1-(2,3-dihydroindol-1-yl)prop-2-en-1-one 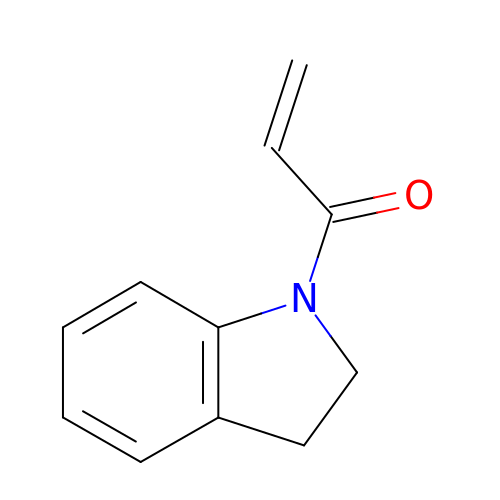| C11 H11 N O | MBODXUXQQPORNR-UHFFFAOYSA-N Here, we reported the enzymatic characterizations and crystal structures of marine bacterial esterases CrmE10 and AlinE4. The results showed that both CrmE10 and AlinE4 belong to the SGNH-hydrolase superfamily and the bacterial lipolytic enzyme GDSL family. The SGNH-hydrolase family, a superfamily that includes the bacterial lipolytic enzyme GDSL family, consists of enzymes possessing four strictly conserved residues, Ser, Gly, Asn, and His, in four conserved blocks, I, II, III, and V, respectively. Among these four residues, Ser and His serve as catalytic residues, and Ser, Gly, and Asn serve as oxyanion hole residues.

In the crystal structure of CrmE10, two identical molecules were found in one asymmetric unit. The CrmE10 structure was composed of 12 α-helices (including three 310-helices) and 5 β-strands. The N-terminal region had a compact architecture that was mainly composed of five predominant β-strands (β1–β5) surrounded by eight α-helices (α1–α8). The C-terminal region was a long α-helix, α9 (Ala184–Asp203), that extended away from the subunit core and wrapped in the other chain. In CrmE10 and AlinE4 structures, catalytic residue Ser was located on helix α1, and residues Asp and His were located on the loop between helix η3 (CrmE10) or helix η2 (AlinE4) and helix α9, which were typically different from other esterases. Interestingly, the catalytic triads of CrmE10 and AlinE4 were not composed of Ser, Asp, and His from the same chain, which was common in other esterases. As mutants CrmE10-S29A and CrmE10-D178A had no activity, the results showed that residues Ser29 and Asp178 influenced the enzymatic activity of CrmE10 by domain swapping. Thus, dimerization participated in the active sites of CrmE10, and this mechanism might also fit AlinE4 due to the similar architecture, which was different from other homologs. The region of these five sites in CrmE10 formed a negative potential surface; however, the corresponding region was full of positive potential in AlinE4. CrmE10 had about 30% activity at 4 °C and showed no activity above 40 °C, which indicated that CrmE10 was a cold-active enzyme.

>MADGEAAGQQADAVMPTGPAIDVLAFGDSLFAGYRLDRDESYPARLQAALRERGLNVNVTNAGVSGDTTAAGLQRIDFVLDSMAGEPDLVLLELGANDMLRGLPAEEARRNLDTILQRLDQRDIPVMVYGMRAAPNLGGDYGRSFDSIFPDLADKYDAELVPFFIEPLIFDRSLVQQDQLHPTAQGVDAMVEQTVEQVEDRIDDL[2x]(1R,2S,4S,5R)-6-(hydroxymethyl)cyclohexane-1,2,3,4,5-pentol 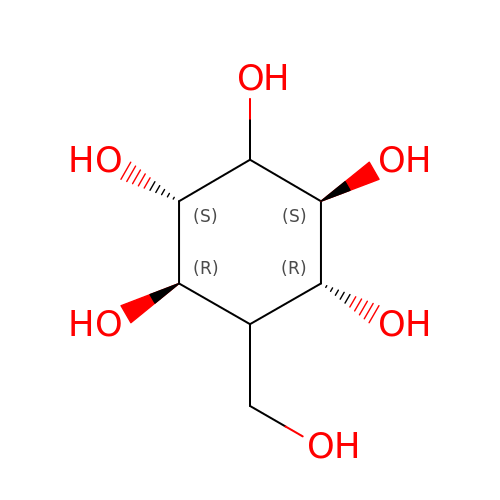| C7 H14 O6 | QFYQIWDMMSKNFF-MAFUWASYSA-N The prototypical systems used to study sequential RNA assembly are group II introns, another class of highly-conserved self-splicing ribozymes of biomedical and bioengineering relevance. Group II introns are validated drug targets for antifungal antibiotics, potentially powerful vectors for genetic engineering, and the evolutionary ancestors of the catalytic RNA core of the eukaryotic spliceosome. Integrating single-particle electron cryomicroscopy (cryo-EM), image processing, in solution small-angle X-ray scattering (SAXS), EM-driven molecular dynamics (MD) simulations, structure-based mutagenesis, and enzymatic assays, we have visualized the sequential multidomain assembly of a self-splicing ribozyme of biomedical and bioengineering significance. Our work reveals a distinct dynamic interplay of helical subdomains in the ribozyme’s 5’-terminal scaffold, which acts as a gate to control the docking of 3’-terminal domains.

All these assembly intermediates are catalytically inactive as they lack the active site residues contributed by D521. E Density of the “partly open” state of D1-4 at 7.05 Å resolution. One conformation, hereafter referred to as the “partly open” state, displays a distinct orientation of ‘peripheral D1c’, which differs clearly from the “catalytic” state despite laterally flanking i1-i2 and D2. Finally, in the D1-4 dataset, we can observe density for D2 and D3, but not for D4, in the “partly open” state. D3 only docks onto D1 in the D1-4 constructs, where however, D4 remains flexible and does not establish tertiary interactions with the rest of the molecule. In line with these chemical probing data, here we show that θ-θ’ is not stably formed in the “open” conformations of D1-2, D1-3, and D1-4.

> GGGGUUAUGUGUGCCCGGCAUGGGUGCAGUCUAUAGGGUGAGAGUCCCGAACUGUGAAGGCAGAAGUAACAGUUAGCCUAACGCAAGGGUGUCCGUGGCGACAUGGAAUCUGAAGGAAGCGGACGGCAAACCUUCGGUCUGAGGAACACGAACUUCAUAUGAGGCUAGGUAUCAAUGGAUGAGUUUGCAUAACAAAACAAAGUCCUUUCUGCCAAAGUUGGUACAGAGUAAAUGAAGCAGAUUGAUGAAGGGAAAGACUGCAUUCUUACCCGGGGAGGUCUGGAAACAGAAGUCAGCAGAAGUCAUAGUACCCUGUUCGCAGGGGAAGGACGGAACAAGUAUGGCGUUCGCGCCUAAGCUUG Here, we identified three N-methyltransferases involved in the biosynthesis of caffeine from the leaves of Kucha. Combined with enzymatic study and kinetic analysis, we found that one of the N-methyltransferases, CkTcS, serves as the critical N9-methyltransferase, which only acts on 1,3,7-trimethyluric acid but not caffeine, indicating that C8-oxidation must take place prior to N9-methylation. The structural characterization of CkTcS identified key residues around the substrate binding pocket that are critical for N9-methyltransferse activity. A previous study using 14C labeled caffeine has confirmed that theacrine is biosynthesized from caffeine, possibly initiated by oxidation at C8 to yield the intermediate 1,3,7-trimethyluric acid followed by N9-methylation.

To explain the substrate specificity of CkTcS, we determined the crystal structure of CkTcS in complex with 1,3,7-trimethyluric acid, in the presence of S-adenosyl-L-homocysteine (SAH), a byproduct of the cofactor SAM, at a resolution of 3.14 Å. Like the coffee methyltransferases, CkTcS exists as a homodimer, and this dimeric arrangement is preserved in the crystal lattice, with the dimer interface composed predominantly of hydrophobic interactions in the core region surrounded by hydrogen bonding interactions. Each monomer of the CkTcS complex consists of a core SAM-dependent methyltransferase domain and a short α-helical cap domain, both of which are involved in the binding of SAH and 5. The major structural difference between the coffee and CkTcS N-methyltransferases occurs on a helix (residues 236-255 in CkTcS), which contributes to the formation of the substrate binding pocket. In CkTcS, this helix is bent with the end close to the substrate moved away from the pocket. The 1,3,7-trimethyluric acid is enveloped in the active site through both hydrogen bonding and van der Waals interactions, with N-9 approximate to the thioether moiety of SAH. The O-6 carbonyl group of 5 is recognized by the Nε groups of Arg-226 through hydrogen-bonds; the side-chain of Trp-161 and His-160 form direct hydrogen bonds with the O-2 carbonyl group of 5. Particularly, the hydroxyl group of Thr-31 forms hydrogen bonds with both N-9 and O-8. The Thr-31-O-8 hydrogen bond may stabilize the O-8 carbonyl group in an iminol tautomeric state, which could facilitate attack of SAM for N9-methylation. Additionally, Phe-322 and Tyr-157 together sandwich the purine ring of 5 through a π–π-stacking interaction.

>SVKEVLFMNTGEGESSYVQNSSFTEKVASMAMPALENAVETLFSKDFHLFQAINAADLGCATGPNTFAVISTIKRMMEKKCRELNCQTLELQVYMNDLFGNDFNTLFKGLSSKVIGNKCEEVSCYVMGVPGSFHGRLFPRNSLHLVHSSYSVHWLTQAPKGLTSREGLALNKGRIYISKTSPPVVREAYLSQFHEDFTMFLNARSQEVVPNGCMVLILRGRQSSDPSDMQSCFIWELLAIAIAELVSQGLIDEDKLDTFNIPCYFPSLEEVKDIVERDGSFTIDHMEGFELDSLQMQENDKWVRGEKFAKIVRAFTEPIISNQFGHEIMDKLYDKFTHIVVSDLEAKLPKTTSIILVLSKIVG[8x]> IAPLVGVGLAAGAVGVGWALREFEIVGSDAPPEGLTADALKQQVYQTAKTRKSTNASTIVDNQNILDGVKHTAYTDAKIAAIEELNAGSAESAVLDAATTEVNSYLTTVQSNFLKTWNESVAELDSILSTVVNHPDIGKGDVFLMLNGSDNTIEDLLANPSGSTDATSFTLADGTTMSVGTVEVDRGTESYYYDPMSGLVGDLGDLKNGGPTVQYDGDSLVYLNASNWKPIYDEMDTVLQNVRSGISTWVSNVYGDVQSGEIEVSDLVTPRERAAMMAQEEGMSQAIADLIALNVPVDAEREATITIQDTGATLPGTFALTDASDGPLESGKTYDPSTFSGDVYFTADMSLVEGDWTAYQSGVDGGNVTLTSEPYSGTAVELNTAANETVAVDAGNWTATGNGTWYHDVSPELETDITSIESARFLSTAEQTQYETIQLQGSFTIDKLTNTQTGEEVTATSFDSSEPHTDSNYITQEEWDQLEQQNKELIEKYEQSQSGGGLDLGQFDMFGIPGEIVAVGVAALVGLGVLGNN

Haloarchaeal pleomorphic viruses (HRPVs) infect archaeal hosts living in hypersaline environments. The virions contain two major protein species, a spike protein (VP4 and VP4-like proteins) protruding from the membrane surface and a smaller membrane associated protein (VP3 and VP3-like proteins) residing mostly inside the virion. Here we describe crystallographic structures of VP4-like spike proteins from two pleolipoviruses, HRPV-2 and HRPV-6, showing that these proteins have a unique fold, different from class I–III fusion proteins. VP5 is thus a bona fide fusion protein.

In order to characterize the VP4-like fusion proteins (termed VP5 in these viruses) from HRPV-2 and HRPV-6, we purified them from infection-competent virions using either detergent (HRPV-2) or protease digestion (HRPV-6). After protein purification, we determined the structures of the HRPV-2 and HRPV-6 VP5 ectodomains (residues 1-498 out of 533 residues and 9-498 out of 537 residues) at 2.5 and 2.7 Å resolution, respectively, by X-ray crystallography. The two proteins, which are 67% identical in amino acid sequence, share a highly conserved V-shaped fold (r.m.s.d. for 453 corresponding Cα atoms: 1.6 Å). The structure is composed of two elongated domains roughly equal in size and linked by a single residue (Q258 in HRPV-2 and Q262 in HRPV-6). In contrast, HRPV-2 VP5 was released intact from the virion by detergent treatment. However, the last 35 residues are not visible in the electron density. The first twenty N-terminal residues of both VP5s are hydrophobic and predicted, by several programs for analysing hydrophobic regions of proteins, to form a transmembrane helix, indicating the preference of this region to partition into membranes. Interestingly, this hydrophobic segment is shielded from the solvent in both crystal structures by the C-terminal domain. HRPV-2 and HRPV-6 VP5 proteins share an average 67% amino acid sequence identity with the N2 subdomain being the least conserved between the two spike proteins. HRPV-2 and -6 infect different host strains suggesting that domain N2 may play a role in host recognition.>MHAALSTEVVHLRQRTEELLRCNEQQAAELETCKEQLFQSNMERKELHNTVM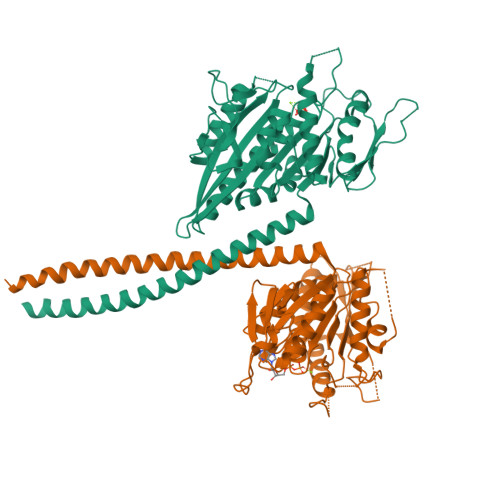DLRGNIRVFCRIRPPLESEENRMCCTWTYHDESTVELQSIDAQAKSKMGQQIFSFDQVFHPLSSQSDIFEMVSPLIQSALDGYNICIFAYGQTGSGKTYTMDGVPESVGVIPRTVDLLFDSIRGYRNLGWEYEIKATFLEIYNEVLYDLLSNEQKDMEIRMAKNNKNDIYVSNITEETVLDPNHLRHLMHTAKMNRATASTAGNERSSRSHAVTKLELIGRHAEKQEISVGSINLVDLAGSESPKTSTRMTETKNIKRSLSELTNVILALLQKQDHIPYRNSKLTHLLMPSLGGNSKTLMFINVSPFQDCFQESVKSLRFAASVNSCKMTKAKRNRYLNNSVANSSTQSNNSGSFDK[2x]> GSHNMTQFEERHLKFLQQLGKGNFGSVEMCRYDPLQDNTGEVVAVKKLQHSTEEHLRDFEREIEILKSLQHDNIVKYKGVCYSAGRRNLK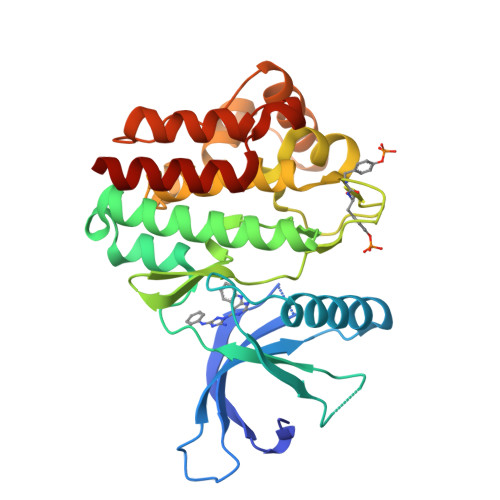LIMEYLPYGSLRDYLQKHKERIDHIKLLQYTSQICKGMEYLGTKRYIHRDLATRNILVENENRVKIGDFGLTKVLPQDKEYYKVKEPGESPIFWYAPESLTESKFSVASDVWSFGVVLYELFTYIEKSKSPPAEFMRMIGNDKQGQMIVFHLIELLKNNGRLPRPDGCPDEIYMIMTECWNNNVNQRPSFRDLALRVDQIRDNMAG>[2x]MAHHHHHHVGTNTGGVLVITDTIIVKSGQTYDGKGIKIIAQGMGDGSQSENQKPIFKLEKGANLKNVIIGA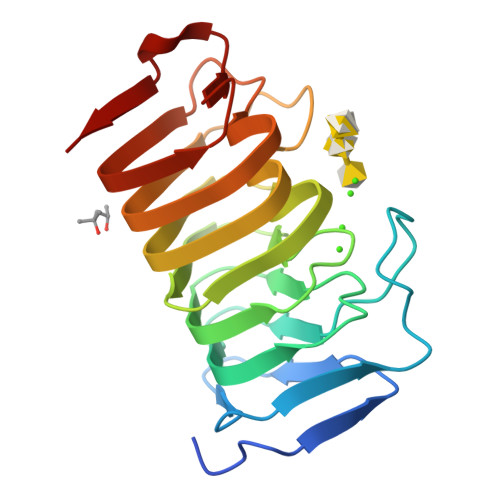PGCDGIHCYGDNVVENVVWEDVGEDALTVKSEGVVEVIGGSAKEAADAVFQLNAPCTFKVKNFTATNIGKLVRQNGNTTFKVVIYLEDVTLNNVKSCVAKSDSPVSELWYHNLNVNNCKTLFEFPSQSQIHQY> PEVGELIEKVRKAHQETFPALCQLGKYTTNNSSEQRVSLDIDLWDKFSELSTKCIIKTVEFAKQLPGFTTLTIADQITLLKAACLDILILRICTRYTPEQDTMTFSDGLTLNRTQMHNAGFGPLTDLVFAFANQLLPLEMDDAETGLL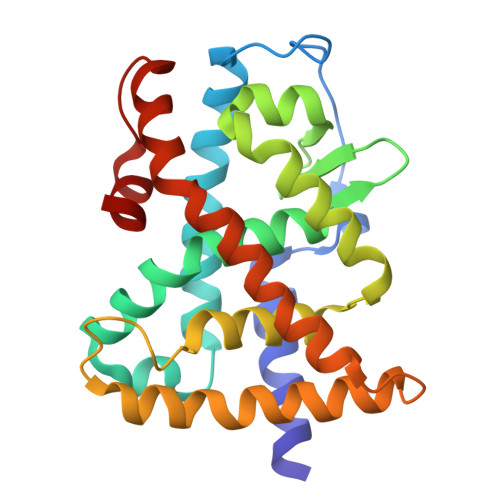SAICLICGDRQDLEQPDRVDMLQEPLLEALKVYVRKRRPSRPHMFPKMLMKITDLRSISAKGAERVITLKMEIPGSMPPLIQEMLE> MDFTKPETVLNLQNIRDELVRMEDSIIFKFIERSHFATCPSVYEANHPGLEIPNFKGSFLDWALSNLEIAHSRIRRFESPDETPFFPDKIQKSFLPSINYPQILAPYAPEVNYNDKIKKVYIEKIIPLISKRDGDDKNNFGSVATRDIECL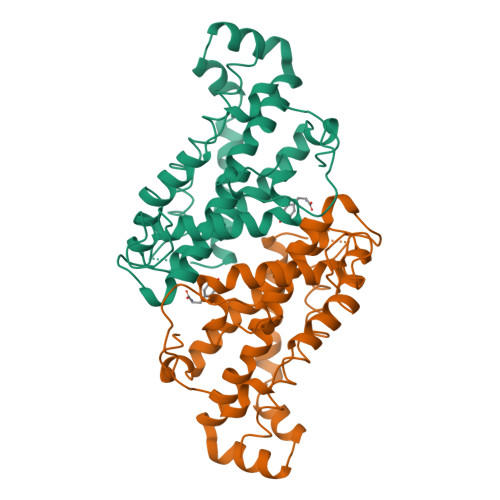QSLSRRIHFGKFVAEAKFQSDIPLYTKLIKSKDVEGIMKNITNSAVEEKILERLTKKAEVYGVDPTNESGERRITPEYLVKIYKEIVIPITKEVEVEYLLRRLEE> MANNWTDILAASDGDEWAAFKTIEAQADEVRAGHQALRRAKPLIRLWMNNPDGSEGLVYVGRVDYDDTIRGSFPFKNNTPSQGVLELRDDNYLAVWLKQLPNNPELKKNVVITVDFYGGKKRWSGLLDKWTIKSKEHVKYLEVTFNDDLTMLQYLLCPPNPALPIPVLQFPRIFGIAGPAKWAISTLIFINLFRVQGNLWTLPDDPFNLESWDDILDWSDWQCFVKSNSFLLDDSSVWTFLSSRMNPVDSIIADALDDAQLTITYRRVLTDDGETAEGFPGAHGIKNGALVFEIVDNSNA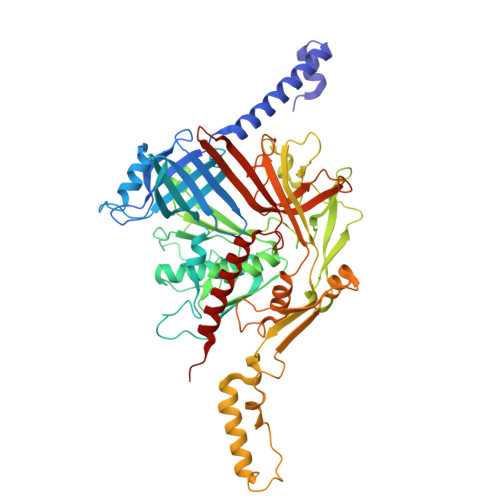TALEGTFFSGTIVDGFARSVLLYGGGFVEDTLSVVSDDQTLQPDEYYQSGWLATMAKMPWLVVRDNEWTPIESSDLSWGPAKNVSVIVGGDNPAADAIAKLIIETTGNLLGYFLLGGFSSAGTIAADIIMPFLVGTIAAWLQWKNTGRATELGWVHYWELYQQGAETNSWSLAALAALRGGFLVGRSETVHLMALHDSWIIPGLHIDIGQRMGSTVNSKGVENIVWVNQLEEMTAAWDNSAGQTMPLSWVLKAGKSDRAMSIGERVARLAKKMSEALNNVGVHIVQS> GPGHMEPAK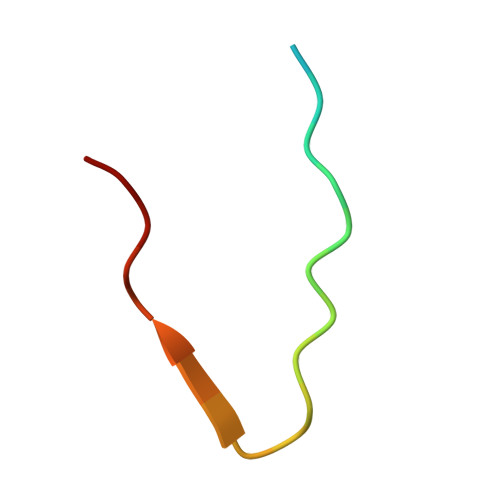LDLPEGQLFFGFPM>[4x]MGNREMEELIPLVNRLQDAFSALGQSCLLELPQIAVVGGQSAGKSSVLENFVGRDFLPRGSGIVTRRPLVLQLVTSKAEYAEFLHCKGKKFTDFDEVRLEIEAETDRVTGMNKGISSIPINLRVYSPHVLNLTLIDLPGITKVPVGDQPPDIEYQIREMIMQFITRENCLILAVTPANTDLANSDALKLAKEVDPQGLRTIGVITKLDLMDEGTDARDVLENKLLPLRRGYVGVVNRSQKDIDGKKDIKAAMLAERKFFLSHPAYRHIADRMGTPHLQKVLNQQLTNHIRDTLPNFRNKLQGQLLSIEHEVEAYKNFKPEDPTRKTKALLQMVQQFAVDFEKRIEGSGDQVDTLELSGGASINRIFHERFPFEIVKMEFNEKEL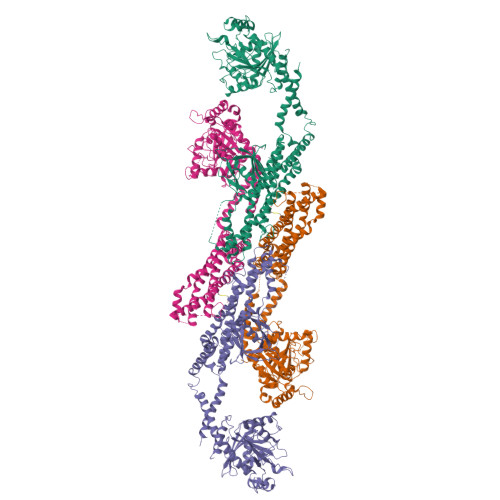RREISYAIKNIHGIRTGLFTPDMAFEAIVKKQIVKLKGPSLKSVDLVIQELINTVKKCTKKLANFPRLCEETERIVANHIREREGKTKDQVLLLIDIQVSYINTNHEDFIGFANAQQRSSQVHKKTTVGNQVIRKGWLTISNIGIMKGGSKGYWFVLTAESLSWYKDDEEKEKKYMLPLDNLKVRDVEKSFMSSKHIFALFNTEQRNVYKDYRFLELACDSQEDVDSWKASLLRAGVYPDKSVAENDENGQAENFSMDPQLERQVETIRNLVDSYMSIINKCIRDLIPKTIMHLMINNVKDFINSELLAQLYSSEDQNTLMEESAEQAQRRDEMLRMYQALKEALGIIGDISTATVSTPAPPPVDDSWIQ> MNDQPFAWQVASLSERYQEQFDIGAAVEPYQLEGRQAQILKHHYNSLVAENAMKPESLQPREGEWNWEGADKIVEFARKHNMELRFHTLVWHSQVPEWFFIDEDGNRMVDETDPDKREANKQLLLERMENHIKTVVERYKDDVTSWDVVNEVIDDGGGLRESEWYQITGTDYIKVAFETARKYGGEEAKLYINDYNTEVPSKRDDLYNLVKDLLEQGVPIDGVGHQSHIQIGWPSIEDTRASFEKFTSLGLDNQVTELDMSLYGWPPTGAYTSYDDIPAELLQAQADRYDQLFELYEELAADISSVTFWGIADNHQWLDGRAREYNNGVGIDAPFVFDHNYRVKPAYWRIIDLEHHHHHH

Xylanase [EC 3.2.1.8] hydrolyzes the internal β-1,4-linkage of xylan. A GH10 xylanase XynR was identified in the culture broth of TAR-110. GH10 xylanases have a (β/α)8 triose-phosphate isomerase (TIM) barrel fold while GH11 xylanases have a β-jellyroll fold composed of eight β strands. GH10 and GH11 xylanases have two conserved catalytically important E residues in the active site.

We made crystallographic analysis of T315Q. The space group of the crystal was C2. The structure was refined at 1.90 Å resolution. The whole structure of T315Q exhibited no difference compared to WT13 with rmsd of 0.65 Å for 353 Cα atoms. WT had three Ca2+ ions, but T315Q had one Ca2+ ion. In T315Q, the side chain of Q315 protrudes inside, resulting in that the distance of Nε2 from the position where the Ca2+ ion located in WT was 1.8 Å. This suggested that such unfavorable distance (1.8 Å) leaded to the steric hindrance between the Nε2 of Q315 and the Ca2+ ion, resulting in the lack of the Ca2+ ion in T315Q. In conclusion, the alkaliphilic XynR variant T315Q lacked the Ca2+ ion near position 315 by keeping the interaction with three of four ligating residues with the Ca2+ ion. Our results suggested that T315Q, and presumably T315H, T315N, and T315S, obtained higher alkaliphily by decreasing stability accompanied by the loss of this Ca2+ ion and the resulting loop (residues 311–331) deviation.> XDPPLHS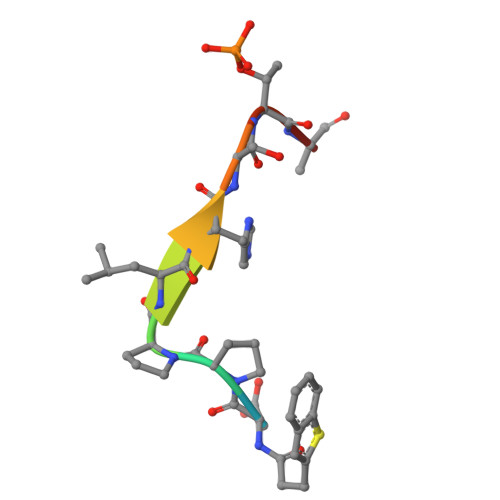TAX>[2x]MSYPYYIVDAFAEEVFKGNPAAVYVLEKWLPEAVMQNIAIENNLSETAFTVKEGQSYALRWFTPEREIDLCGHATLATAFVLFNYYSVAE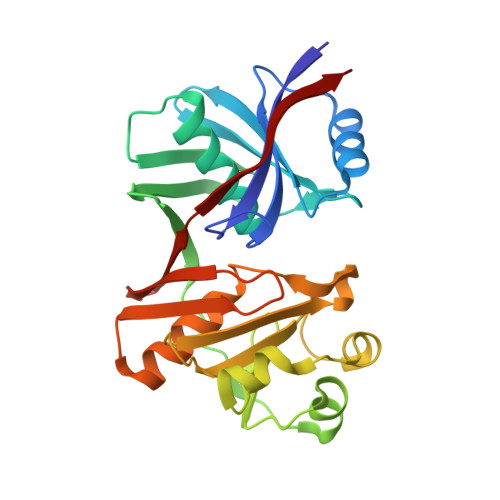ETLHFTSQSGPLAVTKKEEYYYLDFPYILPERIPILPEYEAALGTKIYEAYLGRDLFFVLKDEETVAKITPDFSALKALDLGVGVIVTASGDSVDFVSRTFFPKLRINEDPVCGSAHANLIPYWGKRLNQTTLSAYQVSPRGGFLTCEVKENRVIIGGTAKLFAKGEAYLPV> MIQQMDQYISMQNESSSEISDIETRSPSHSFEDNLKYYSDIYEVLSKDQIKQEYEQLQKSNFVKNIIRSFYLFILESGDEIVIESMFENQEKGIIQIRKEFQT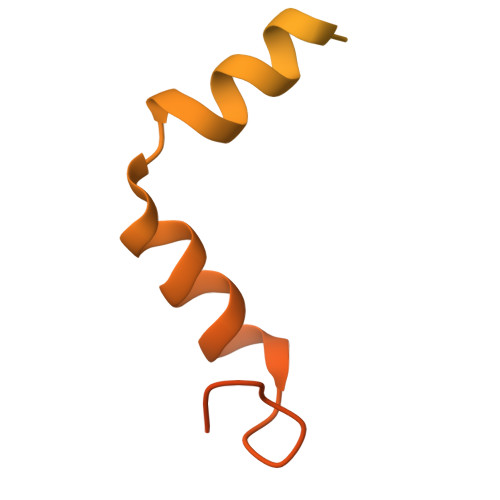FTRQKKFNQSTLNSLINSKRFGKIFYYFLKYYIYDWVISRSVKDLKSHVIFITYLKKQLEQNIENQQFD>[2x]MSDTMVVNGSGGVPAFLFSGSTLSSYRPNFEANSITIALPHYVDLPGRSNFKLMYIMGFPIDTEMEKDSEYSNKIRQE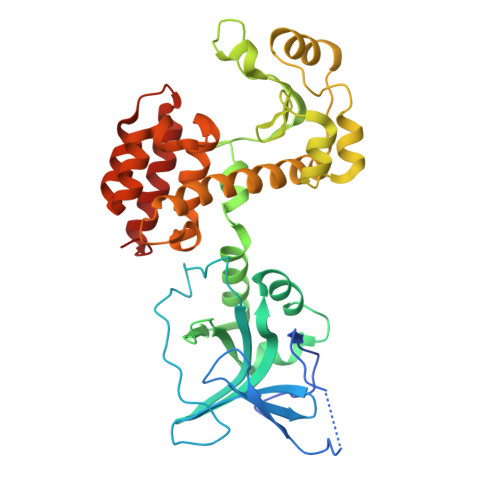SKISKTEGTVSYEQKITVETGQEKDGVKVYRVMVLEGTIAESIEHLDKKENEDILNNNRNRIVLADNTVINFDNISQLKEFLRRSVNIVDHDIFSSNGFAGFNPTSHFPSNPSSDYFNSTGVTFGSGVDLGQRSKQDLLNDGVPQYIADRLDGYYMLRGKEAYDKVRTAPLTLSDNEAHLLSNIYIDKFSHKIEGLFNDANIGLRFSDLPLRTRTALVSIGYQKGFKLSRTAPTVWNKVIAKDWNGLVNAFNNIVDGMSDRRKREGALVQKDIDSGLLK> TQAKAKHADVPVNLYRPNAPFIGKV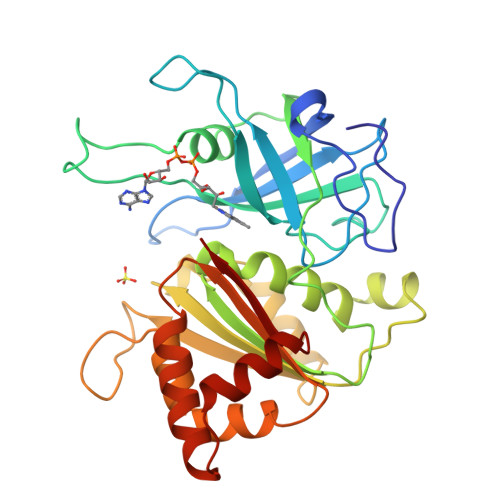ISNEPLVKEGGIGIVQHIKFDLTGGNLKYIEGQSIGIIPPGVDKNGKPEKLRLYSIASTRHGDDVDDKTISLCVRQLEYKHPESGETVYGVCSTYLTHIEPGSEVKITGPVGKEMLLPDDPEANVIMLATGTGIAPMRTYLWRMFKDAERAANPEYQFKGFSWLVFGVPTTPNILYKEELEEIQQKYPDNFRLTYAISREQKNPQGGRMYIQDRVAEHADQLWQLIKNQKTHTYICGLRGMEEGIDAALSAAAAKEGVTWSDYQKDLKKAGRWHVETY> GAMGSDFEEWISGTYRKMEEGPLPLLTFATAPYHDQKPGTSGLRKKTYYFEEKPCYLENFIQSIFFSIDLKDRQGSSLVVGGDGRYFNKSAIETIVQMAAANGIGRLVIGQNGILSTPAVSCIIRKIKAIGGIILTASHNPGGPNGDFGIKFNISNGGPAPEAITDKIFQISKTIEEYAVCPDLKVDLGVLGKQQFDLENKFKPFTVEIVDSVEAYATMLRSIFDFSALKELLSGPNRLKIRIDAMHGVVGPYVKKILCEELGAPANSAVNCVPLEDFGGHHPDPNLTYAADLVETMKSGEHDFGAAFDGDGDRNMILGKHGFFVNPSDSVAVIAANIFSIPYFQQTGVRGFARSMPTSGALDRVASATKIALYETPTGWKFFGNLMDASKLSLCGEESFGTGSDHIREKDGLWAVLAWLSILATRKQSVEDILKDHWQKYGRNFFTRYDYEEVEAEGANKMMKDLEALMFDRSFVGKQFSANDKVYTVEKADNFEYSDPVDGSISRNQGLRLIFTDGSRIVFRLSGTGSAGATIRLYIDSYEKDVAKINQDPQVMLAPLISI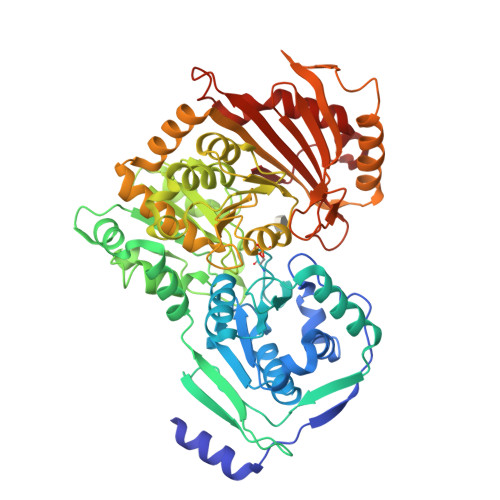ALKVSQLQERTGRTAPTVIT>[2x]MASQGPGEVVLLDFAAA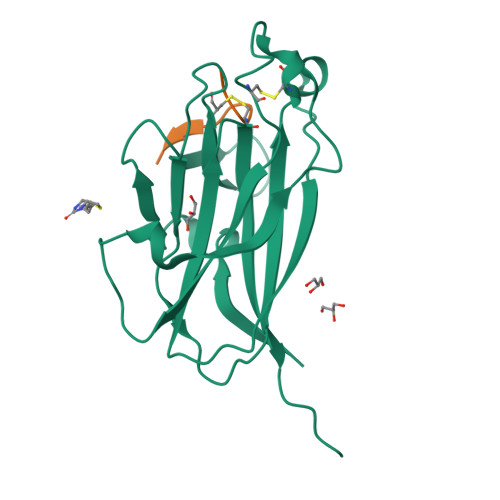GGELGWLTHPYGKGWDLMQNIMNDMPIYMYSVCNVMSGDQDNWLRTNWVYRGEAERIFIELKFTVRDCNSFPGGASSCKETFNLYYAESDLDYGTNFQKRLFTKIDTIAPDEITVSSDFEARHVKLNVEERSVGPLTRKGFYLAFQDIGACVALLSVRVYYKKAHHHHHH;>YSAYPDSVPMMSGSGSK[2x]> MKDIAIRGYCDRPSVATGETIRFYVSANETRGTFDAELVRLIHGDSNPAGPGYKEEAIKSDLEGQYPARFQRTQFGSYVEVADPDAGLQPDGAFSVHLFLWSTTPSRGRQGIASRWNDERQSGWNLAIEDGRVVFTIGDGSGATSSVVSDRPLFQQIWYSITGVYDPEKKQLRLYQKSVVNRTNSRFGLVVPLDSDCAVSADATVKAADSETSLLIAGLGEAAAQDGRTWCIAHYNGKVDAPKIYGCALGQDDAEKLSRGEIVRPISRLAHWDFSAGIGLNGIPTDHVVDASGYGHHGRCMNQPSRGSTGWNWDGHEENFIHCPEQYGALWFHEDCLDDCRWEKDFEFTVPEGLKSDFYAVKIRYEDTEDYIPFFVLPPRGTATAPILVIASTLSYLAYANEQIMHKADIGQAVAGHTPVLNENDVELHKNLSYYGLSTYDGHIDGRGVQYTSWRRPIMNLRPKHRQGFGSIWELPADLHLIDWLNHNGFEYDVATEHDLNDQGAELLR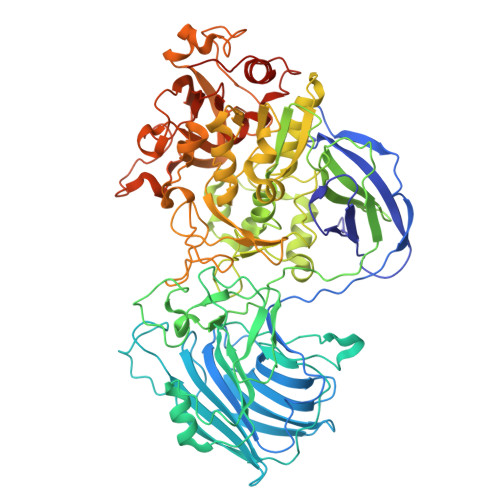RYKVVLTGSHPEYQTWANADAWEDYLADGGRGMYLAANGMYWIVEVHPEKPWVMEVRKELGVTAWEAPPGEYHYSTNGRRGGRFRGRARATQKIWGTGMSSFGFDHSGYFVQMPDSQDERVAWIMEGIDPEERIGDGGLVGGGAGGYELDRYDLALGTPPNTLLLASSVEHSVVYTVIPDDKAFPHPGMNGGEHPFVRADITYFSTANGGGMFATSSISWLGSLSWNDYDNNVSKMTKNVLNQFIKDEPAPRVKLAAALEHHHHHH>[2x]HHHHHHSSGLVPRGSHMETESLPWREYLERIGYQGLLNNSLECLRELYTAHLRSVPYEMLDSFDGTPPVLGHAESFAKLVHRRRGGNCLESTPLFGEFLRQAGFEVRLVPAQIWKVSGEWWDAWDHLLLIVTVDGEDWLLDVGFLMLTFAEPLKVAEGP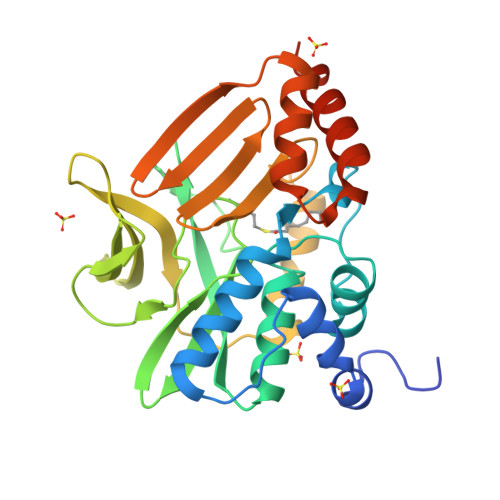QEQSGWRFRVAEEEGFPTVSHQGPDGTWTAVYRYRDEPQQRADYEWIIDFHKSAEDSPLVGTLLCSRNVPDGKLIMIGENLLHARNGRVSAEFIETTSRAEELLRVIFAGHEHMVESAVRTWEKARADRSTRRSLVYRKAEQ>[4x]GSARQQEIDMKRQQRFFRIPFIRPADQYKDPQNKKKGWWYAHFDGPWIARQMELHPDKPPILLVAGKDDMEMCELNLEETGLTRKRGAEILPRQFEEIWERCGGIQYLQSAIES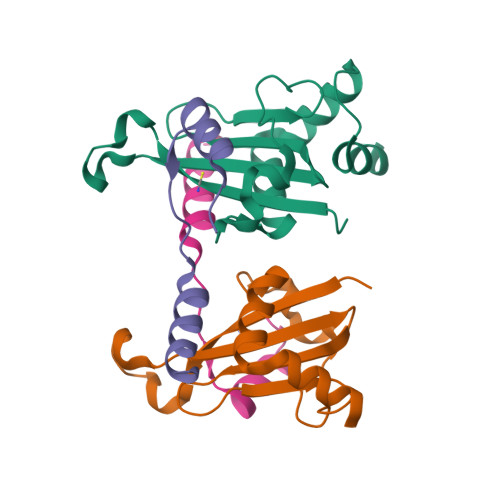RQARPTYATAMLQNLLKGSSGGSLVPR;>GSSSGGGSSSSGTSSAFSSYFNNKVGIPQEHVDHDDFDANQLLNKINE[4x]The TRAPP complexes are nucleotide exchange factors that play essential roles in membrane traffic and autophagy. TRAPPII activates Rab11, and TRAPPIII activates Rab1, with the two complexes sharing a core of small subunits that affect nucleotide exchange but being distinguished by specific large subunits that are essential for activity in vivo. We report a cryo‐EM structure of the entire Drosophila TRAPPIII complex. The TRAPPIII‐specific subunits TRAPPC8 and TRAPPC11 hold the catalytic core like a pair of tongs, with TRAPPC12 and TRAPPC13 positioned at the joint between them.

However, in the regions of TRAPPC8 and TRAPPC11 located on either side of the core the local resolution was suitable for de novo model building. In the case of TRAPPC8, residues 350–660 form an α‐solenoid of thirteen α‐helices that includes the site of interaction with TRAPPC2. TRAPPC8 (yellow) is formed by thirteen α‐helices and binds TRAPPC2 via helices 9, 10 and 11. The less well‐resolved C‐terminal region (residues 660–1,319) forms the arm that connects to TRAPPC12 and TRAPPC13. This part of TRAPPC8 is not present in the yeast orthologue Trs85, consistent with it forming an armless complex. The interaction between TRAPPC2 and TRAPPC8 encloses a total surface area of ~550 Å with the TRAPPC2‐binding region of TRAPPC8 formed by α‐helices 9 and 11. Conserved regions in TRAPPC8 (Pro559‐His567 in α‐helix 9 and Trp600‐Ile607 in α‐helix 11) form a hydrophobic pocket needed for the interaction. In addition, α‐helix 9 contains several polar and charged residues, such as Arg562 and Lys563, that are likely to interact with key residues in TRAPPC2, including Asp46. Interestingly, Asp46 appears to be particularly critical for the assembly of TRAPP complexes as mutation of this residue causes spondyloepiphyseal dysplasia tarda in humans and disrupts the TRAPP complexes in yeast.

> DNLRHFVQDYAVRALIPYIEHLVAILAEGVTNKKGVSKSLLSATKRWFVTSKPGAGANNQNAVIYTNESAELQTRKLGDLYFMFGHYNLAFQSYHQAKRDFNADSAWQYYAGALEMAALSAFMLGTAQRKTYDYMEDAIVCYLTVCKLQQFATRATLLSMECLKTARLYSEVAKQLIRMTNEESDLRSALLLEQAAYCFLVTQPPMHRKYAFHIVLAGNRYSRAGQRKHAYRCYRQAYQVFQKREWSLAEDHIQYTVAKQAYMLKQLEEASRSFAHLLRPGSLQSAQQQTSFLKEYIQTQNELVKRS>KVTYTSQEDLVEKKCLAKKYTHLSCDKVFCQPWQRCIEGTCVCKLPYQCPKNGTAVCATNRRSFPTYCQQKSLECLHPGTKFLNNGTCTAEGKFSVSLKHGNTDSEGIVEVKLVDQDKTMFICKSSWSMREANVACLDLGFQQGADTQRRFKLSDLSINSTECLHVHCRGLETSLAECTFTKRRTMGYQDFADVVCYTQKADSPMDDFFQCVNGKYISQMKACDGINDCGDQSDELCCKACQGKGFHCKSGVCIPSQYQCNGEVDCITGEDEVGCAGFASVAQEETEILTADMDAERRRIKSLLPKLSCGVKNRMHIRRKRIVGGKRAQLGDLPWQVAIKDASGITCGGIYIGGCWILTAAHCLRASKTHRYQIWTTVVDWIHPDLKRIVIEYVDRIIFHENYNAGTYQNDIALIEMKKDGNKKDCELPRSIPACVPWSPYLFQPNDTCIVSGWGREKDNERVFSLQWGEVKLISNCSKFYGNRFYEKEMECAGTYDGSIDACKGDSGGPLVCMDANNVTYVWGVVSWGENCGKPE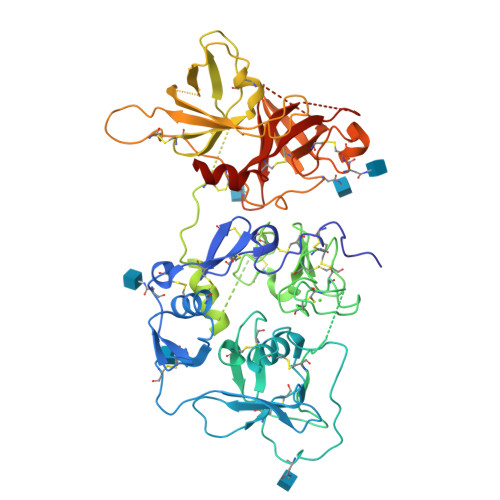FPGVYTKVANYFDWISYHVGRPFISQYNV[4x]>[2x]MVQWSPFVMSFKKKYPWIQLAGHAGSFKAAANGRILKKHCESEQRCLDRLMADVLRPFVPAYHGDVVKDGERYNQMDDLLADFDSPCVMDCKMGVRTYLEEELTKARKKPSLRKDMYQKMVEVDPEAPTEEEKAQRAVTKPRYMQWRETISSTATLGFRI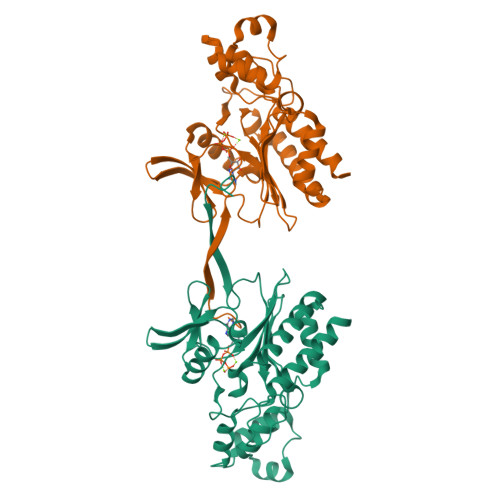EGIKKEDGSVNRDFKKTKTREQVTEAFREFTKGNQNILIAYRDRLKAIRATLEISPFFKCHEVIGSSLLFIHDKKEQAKVWMIDFGKTTPLPEGQTLQHDVPWQEGNREDGYLSGLDNLIDILTEMSQG> MFKTILLAYDGSEHARRAAEVAKAEAEAHGARLIV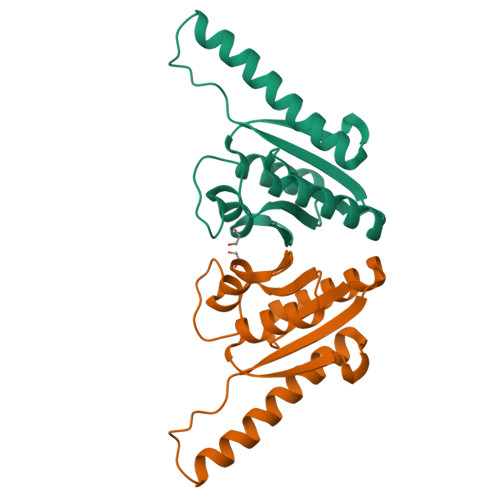VHAYEPVPDYLGEPFFEEALRRRLERAEGVLEEARALTGVPKEDALLLEGVPAEAILQAARAEKADLIVMGTRGLGALGSLFLGSQSQRVVAEAPCPVLLVR> GDTKEQRILRYVQQNAKPGDPQSVLEAIDTYCTQKEWAMNVGDAKGQIMDAVIREYSPSLVLELGAYCGYSAVRMARLLQPGARLLTMEINPDCAAITQQMLNFAGLQDKVTILNGASQDLIPQLKKKYDVDTLDMVFLDHWKDRYLPDTLLLEECG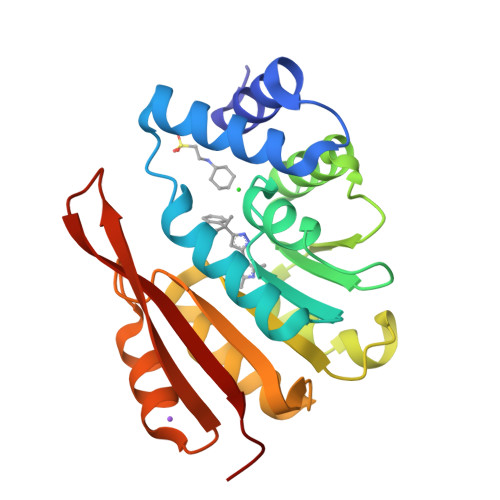LLRKGTVLLADNVIVPGTPDFLAYVRGSSSFECTHYSSYLEYMKVVDGLEKAIYQGPS To evaluate metal-ion affinity and to identify protein metal-binding sites for Sr2+ and Cs+, a class C β-lactamase (BLA) derived from the moderate halophile Chromohalobacter sp. 560 (HaBLA; molecular weight 39 536) was chosen as a model system. HaBLA, although a moderately halophilic periplasmic protein, has a particularly abundant content of acidic amino acids similar to those in extremely halophilic proteins. The crystal structure of a halophilic β-lactamase from Chromohalobacter sp. 560 (HaBLA) was determined to resolutions of between 1.8 and 2.9 Å in space group P31 using X-ray crystallography. Seven binding sites (site 1 to site 7) for divalent metal ions (Ca2+ and/or Sr2+) and one binding site (site 8) for Cs+ per HaBLA molecule were identified by X-ray diffraction studies including anomalous dispersion.

WT-HaBLA crystallized in the presence of Na+ and Mg2+ but without Sr2+ and Cs+. The tertiary structure of WT-HaBLA was determined to 2.9 Å resolution. The solvent content in the WT-HaBLA crystal was 44.6%. The tertiary structure of WT-HaBLA contains 12 α-helices and 16 β-strands, which is the same as in halophilic class C BLAs. In addition, the binding sites for Mg2+ in the structure of WT-HaBLA were not identified because of the noisy electron-density map owing to the low resolution of the X-ray diffraction (2.9 Å). From a structural comparison of these five catalytic residues in WT-HaBLA and EaBLA, only a small side-chain rearrangement of the catalytic residues in WT-HaBLA was found. The r.m.s.d. for side-chain atoms between the active sites of WT-HaBLA and EaBLA was <1.4 Å. The active site was positively charged owing to the existence of Lys68, His113, Arg149 and Lys316 even in the negatively charged circumstances of the overall structure. In the vicinity of the active site of HaBLA, we also found a hydrophobic cluster composed of five hydrophobic and aromatic residues: Leu120, Phe121, Tyr290, Ile293 and Leu294. The side chains of Leu120 and Ile293 of HaBLA form van der Waals contacts (within 4 Å distance) with the aromatic ring of Tyr151 in the active site, as observed in EaBLA.

>QDDASDRQTREVLDPIVASLMEAQQIPGMAIALVRPEGTTISHYGAADRETGTPVDDDTLFEIGSLSKTLTATLASLAEVEGKLDFDAPVSRYLPELEGSAFDDISGLNLGTHTGGGLPLFVPDEVTDRASLMAWYREWQPTEPIGESRTYSNLGIGLLGLETAASLDGEFVPTMRAKVLAPLGMQDTWYDVPEARMADYAMGEDKDGQPTRVSPGVLDDEAYGIKTTAADLAKLVRANLHLADVDAELQQAIDATRQGHYRVGDMTQALIWEQYSLPVAPETLRAGNGYDMILEPNAAEALEPPQSPRDDVWVNKTGSTNGFGGYIVMLPGKHTGLVMLANKNYPNDARVEAAYRILSGLGAIDVP[3x]(1~{R})-7-[(1~{R})-1,2-bis(oxidanyl)ethyl]-1,3-dimethyl-5-(1-methylpyrazol-4-yl)-1~{H}-3-benzazepin-2-one | C18 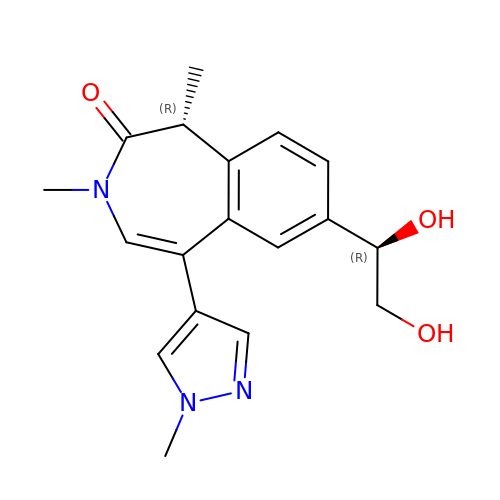H21 N3 O3 | CJVJSGBELMMESS-DIFFPNOSSA-N> NDDKEAKKEAQEKEKNTPNGLVYTNLDFDSFKATIKNLKDKKVTFKEVNPDIIKDEVFDFVIVNRVLKKIKDLKHYDPMIEKIFDEKGKEMGLNVEIQINPEVKDFFTFKSISTTNKQRCFLSLRGETREILCDNKLYNML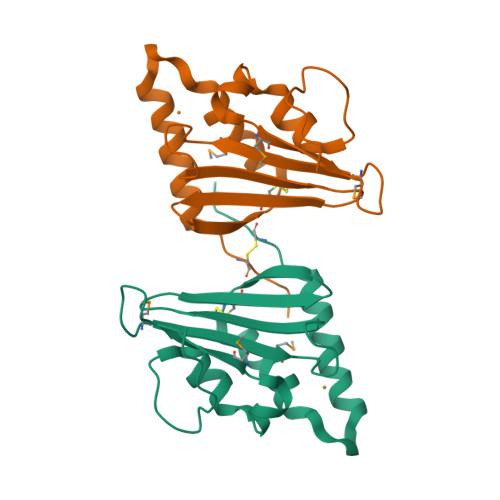LAVFNSYDPNDLLKHISTVESLKKIFYTITCEAVY> GSHMSPSDLHLPVPGHPIAAIATPVGVGALAIVRISGAGVLDLADRVFRKVHGSGKLAEAAGYTAHFGRLYDGEEMVDEVIALVFRAPRSFTAEQMVEFTCHGGPVVVGRVLRLMLDNGCRLAEPGEFTRRAFLNGRIDLLQAEAIGEMIHARTESAYRTAVSQMKGDLSVRLGGLREQLIRSCALIELELDFSEEDVEFQSRDELTMQIETLRSEVNRLIDSYQHGRIVSEGVSTVIAGKPNAGKSTLLNTLLGQERAIVSHMPGTTRDYIEECFIHDKTMFRLTDT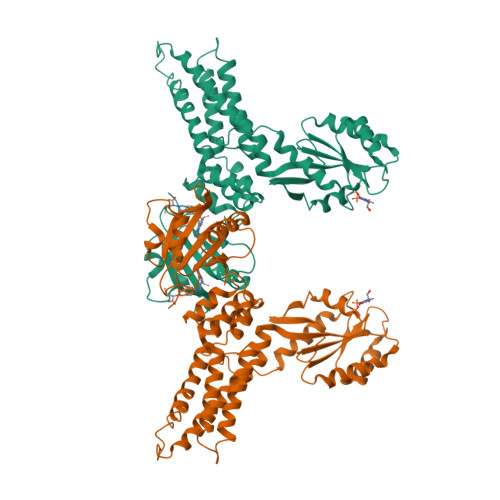AGLREAGEEIEHEGIRRSRMKMAEADLILYLLDLGTERLDDELTEIRELKAAHPAAKFLTVANKLDRAANADALIRAIADGTGTEVIGISALNGDGIDTLKQHMGDLVKNLDKLHEASVLVTSLRHYEALRNASDALQNALELIAHESETELIAFELRAALDYVGQITGKVVNEEVLNTIFDKFCIGK The bacterial P450 OleP, from Streptomyces antibioticus, is an epoxidase involved in the tailoring steps of the biosynthetic pathway of the antibiotic oleandomycin. More specifically, OleP catalyzes a regio- and stereospecific reaction of epoxidation at the C8-C8a of the macrolactone ring. Among the known macrolide epoxygenases from actinomycetes, OleP presents a unique epoxidation chemistry since it targets a non-activated C-C bond, which is a reaction not easily achievable through conventional chemical synthesis protocols. In addition, discordant findings have been reported concerning the timing of OleP activity during the tailoring phase of oleandomycin biosynthesis, showing that OleP is either active on the aglycone intermediate, 8.8a-deoxyoleandolide (DEO), or on the monoglycosylated one, L-olivosyl-8.8a-deoxyoleandolide (L-O-DEO).

The omit maps of the ternary complex structures clearly revealed the presence of a bulky, partially defined, electron density within the solvent cavity of most of the OleP monomers in the asymmetric unit of both crystals. Since this density was absent in the omit maps of the corresponding aglycone-bound OleP crystals where the L-rhamnose was not added, we interpreted it as a molecule of the sugar. However, the freedom of movement of the sugar molecule inside the cavity, which is only limited by sterically prohibited contacts, resulted in poorly defined electron densities of the ligand. Successful refinement gave an average of occupancy of 60% for each identified L-rhamnose molecule. Due to its flexibility, to the absence of chemical linkage to the aglycone and to the available room in the solvent cavity, L-rhamnose adopts different positions, orientations, and conformations inside each monomer, contacting via hydrogen bonds and van der Waals interactions: (i) OleP residues present in the cavity, (ii) the aglycone moiety bound to the active site at C3-OH and C5-OH, and (iii) solvent molecules. Most contacts established in the crystal structures by L-rhamnose with OleP correspond to the ones observed in silico for the glycosyl moiety of docked L-O-DEO. These contacts include E89 and G92 on the BC loop, and N236, V239, S240, and I243 on the I helix. L-rhamnose in the ternary complex establishes contacts with M178 on the F helix and Q193 on the G helix, which were absent in the docking simulation. All the abovementioned residues are located on secondary structural regions that participate in the open-to-closed structural transition.

>MTDTHTGPTPADAVPAYPFSLPHALDLDPHYAELRRDEPVSRVRLPYGEGTAWLVTRMSDARIVLGDSRFSTAAATDPATPRMFPTPPEPDGVLAQDPPDHTRLRRLVGKAFTARRVEEMRPRVRSLVDSLLDDMVAHGSPADLVEFLAVPFPVAVICELLGVPLEDRDLFRTFSDAMLSSTRLTAAEIQRVQQDFMVYMDGLVAQRRDAPTEDLLGALALATDNDDHLTKGEIVNMGVSLLIAGHETSVNQITNLVHLLLTERKRYESLVADPALVPAAVEEMLRYTPLVSAGSFVRVATEDVELSTVTVRAGEPCVVHFASANRDEEVFDHADELDFHRERNPHIAFGHGAHHCIGAQLGRLELQEALSALVRRFPTLDLAEPVAGLKWKQGMLIRGLERQIVSW[6x]> CTMIPQYEQPKVEVAETFQNDTSVSSIRAVDLGWHDYFADPRLQKLIDIALERNTSLRTAVLNSEIYRKQYMIERNNLLPTLAANANGSRQGSLSGGNVSSSYNVGLGAASYELDLFGRVRSSSEAALQGYFASVANRDAAHLSLIATVAKAYFNERYAEEAMSLAQRVLKTREETYNAVRIAVQGRRDFRRRPAPAEALIESAKADYAHAARSREQARNALATLINRPIPEDLPAGLPLDKQFFVEKLPAGLSSEVLLDRPDIRAAEHALKQANANIGAARAAFFPSIRLTGSVGTGSVELGGLFKSGTGVWAFAPSITLPIFTWGTNKANLDVAKLRQQAQIVAYESAVQSAFQDVANALAAREQLDKAYDALSKQSRASKEALRLVGLRYKHGVSGALDLLDAERSSYSAEGAALSAQLTRAENLADLYKALGGGLKRDTQTGK

The best characterized and most clinically important efflux system in N. gonorrhoeae is the MtrCDE tripartite multidrug efflux system, which belongs to the hydrophobic and amphiphilic efflux resistance-nodulation-cell division (HAE-RND) family. The membrane fusion protein MtrC, containing 412 amino acids, bridges MtrD and MtrE to form the tripartite efflux complex MtrCDE. This powerful efflux complex spans the entire cell envelope of N. gonorrhoeae and mediates the export of hydrophobic antimicrobial agents, such as antibiotics, nonionic detergents, antibacterial peptides, bile salts and gonadal steroidal hormones.

MtrE is a 447 amino acid protein that forms an outer membrane channel. Here we present the crystal structure of the outer membrane MtrE channel, which represents an open conformational state of this multidrug efflux protein. The crystal structure of the full-length MtrE outer membrane channel protein was then determined to a resolution of 3.29 Å. Like TolC and OprM, MtrE exists as a homotrimer that forms a ∼130 Å long α/β barrel. Each subunit of MtrE contains four β-strands (contributing to the 12-stranded outer membrane β-barrel) and eight α-helices (forming the elongated periplasmic α-barrel). In view of the crystal structure of MtrE, it is found that the internal surface of the protein forms a continuous channel. This channel is completely open and fully accessible through both the periplasmic end and outer membrane surface, suggesting that the MtrE channel is at its open conformational state. Each protomer of MtrE contributes D402 and D405 to form two concentric circles of negative charges in the inner cavity of the trimeric MtrE channel. The internal diameter of the MtrE aspartate ring is ∼12 Å, which creates the narrowest region of the tunnel. Additionally, the distance between the Cα atoms of these aspartates is 16.0 Å. It is suspected that the open conformational state of MtrE reflects the low-pH form of this channel, as we crystallized this channel at low pH which would neutralize the aspartate ring.>[2x]HMGSEGGPALFQSDMTFK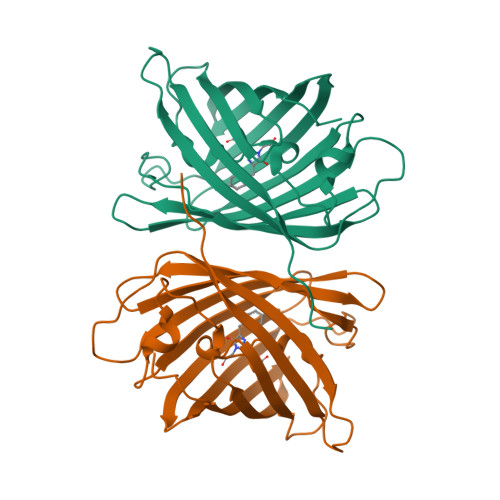IFIDGEVNGQKFTIVADGSSKFPHGDFNVHAVCETGKLPMSWKPICHLIQYGEPFFARYPDGISHFAQECFPEGLSIDRTVRFENDGTMTSHHTYELDDTCVVSRITVNCDGFQPDGPIMRDQLVDILPNETHMFPHGPNAVRQLAFIGFTTADGGLMMGHFDSKMTFNGSRAIEIPGPHFVTIITKQMRDTSDKRDHVCQREVAYAHSVPRITSAIGSDED1-{5-bromo-2-[(3R)-3-hydroxypiperidin-1-yl]phenyl}-3-(5-cyanopyrazin-2-yl)urea 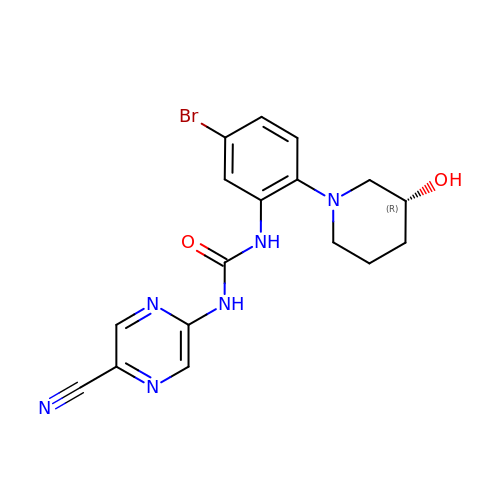| C17 H17 Br N6 O2 | BBKALDDXSCLMBB-CYBMUJFWSA-N>[2x]MIDLSKTVFYTSIDIGSRYIKGLVLGKRDQEWEALAFSSVKSRGLDEGEIKDAIAFKESVNTLLKE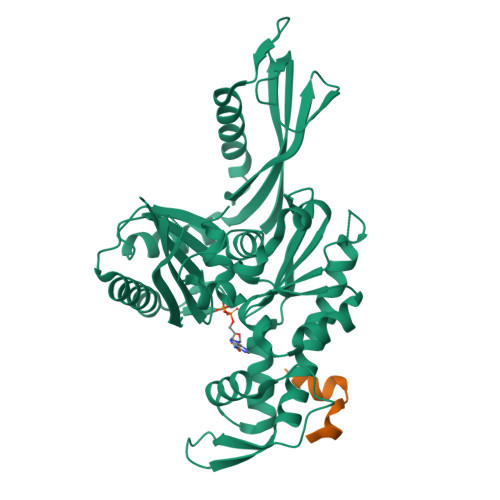LEEQLQKSLRSDFVISFSSVSFEREDTVIERDFGEEKRSITLDILSEMQSEALEKLKENGKTPLHIFSKRYLLDDERIVFNPLDMKASKIAIEYTSIVVPLKVYEMFYNFLQDTVKSPFQLKSSLVSTAEGVLTTPEKDRGVVVVNLGYNFTGLIAYKNGVPIKISYVPVGMKHVIKDVSAVLDTSFEESERLIITHGNAVYNDLKEEEIQYRGLDGNTIKTTTAKKLSVIIHARLREIMSKSKKFFREVEAKIVEEGEIGIPGGVVLTGGGAKIPRINELATEVFKSPVRTGCYANSDRPSIINADEVANDPSFAAAFGNVFAVSENPYEETPVKSENPLKKIFRLFKELME;>EGDIPAIYRYGLEGLL[2x]methyl 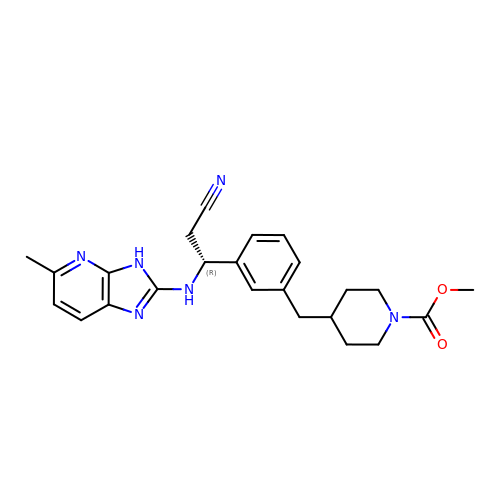4-[(3-{(1R)-2-cyano-1-[(5-methyl-3H-imidazo[4,5-b]pyridin-2-yl)amino]ethyl}phenyl)methyl]piperidine-1-carboxylate | C24 H28 N6 O2 | NAKOGAFXAQIHDB-HXUWFJFHSA-N> ASSMASEVGRRLAEF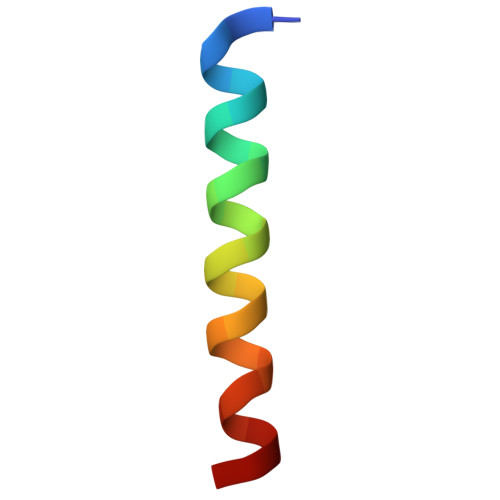GDQVDGQFYQ> GSNDDFTGEDSLMEDHLELREKLSEDIDMIKTSLKNNLVCSTLNDNEILTLSNYMQFFVFKSGNLVIKQGEKGSYFFIINSGKFDVYVNDKKVKTMGKGSSFG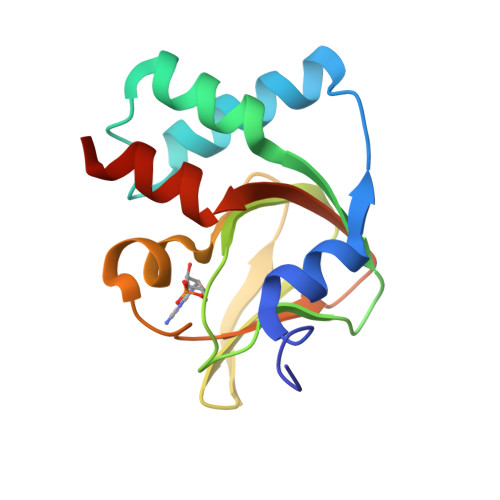EAALIHNTQRSATIIAETDGTLWGVQRSTFRATLKQLSNR>[4x]GSHMEQLKCCSGILKEMFAKKHAAYAWPFYKPVDVEALGLHDYCDIIKHPMDMSTI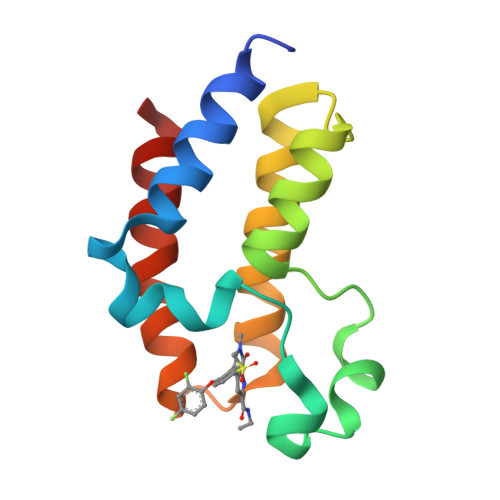KSKLEAREYRDAQEFGADVRLMFSNCYKYNPPDHEVVAMARKLQDVFEMRFAKM> LMGCVAETPPRFTRTPVDQTGVSGGVASFICQATGDPRPKIVWNKKGKKVSNQRFEVIEFDDGSGSVLRIQPLRTPRDEAIYECVASNNVGEISVSTRLTVLREDQIPRGFPTIDMGPQLKVVERTRTATMLCAASGNPDPEITWFKDFLPVDTSNNNGRIKQLRSESIGGTPIRGALQIEQSEE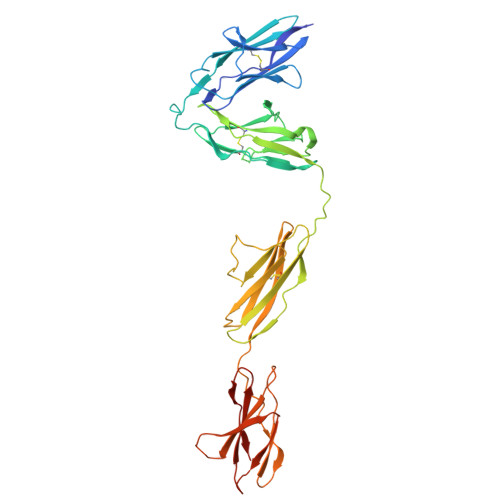SDQGKYECVATNSAGTRYSAPANLYVRELREVRRVPPRFSIPPTNHEIMPGGSVNITCVAVGSPMPYVKWMLGAEDLTPEDDMPIGRNVLELNDVRQSANYTCVAMSTLGVIEAIAQITVKALPKPPGTPVVTESTATSITLTWDSGNPEPVSYYIIQHKPKNSEEPYKEIDGIATTRYSVAGLSPYSDYEFRVVAVNNIGRGPASEPVLTHHHHHH> GVALGATRVIYPAGQKQEQLAVTNNDENSTYLIQSWVENADGVKDGRFIVTPPLFAMKGKKENTLRILDATNNQLPQDRES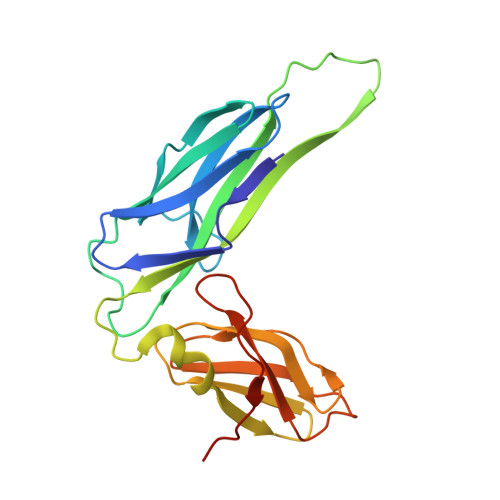LFWMNVKAIPSMDKSKLTENTLQLAIISRIKLYYRPAKLALPPDQAAEKLRFRRSANSLTLINPTPYYLTVTELNAGTRVLENALVPPMGESTVKLPSDAGSNITYRTINDYGALTPKMTGVMEHHHHHH> MYLSFYITDTKNKLIFQYLLGATAPSFKHLWTRVQSTCPQLLEDSSSDDYLDHSMVGRDLEVYKYFSVINKLNYWCLASTSKSKGPLDCFTFLETIDRILLEYFDKDKLSIKKIVNNYDRISLIFNCCVEAGEPNVSDMLYVNKIKEAVPERSDLSKFISSTAHNLQQAVQLPQQRQQQLQQNQISRGSNSLIENEEIVPWRTSRASKHENNELYVDLLETFHVVFEKKKSHLRLLTGSIHGIVDVRSYLNDNPLVAVKLNTMGNDIGIPSLHDCVEINDGVFSPSNITFIPPDGKFRLLEYSVDLSSQVKQSGVRMNSIGLMSLHFQNGLGKDS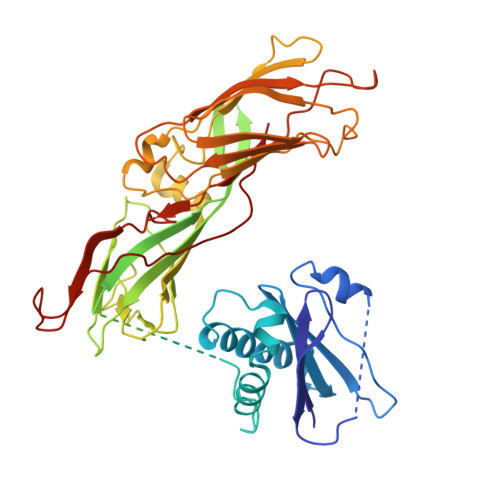DEFELSLNIENFKKVSQVDDLKIDLQFNVENADPNEIAYKIKILRNTHGRFENSIIMGQGQWIFDKSTATGTVPVLRGCIEYENTGPNFTKKVDLQTVSLEYSYIGQSASGIYVEAIDIVSGLTIGKNTKLYKGAKYKTQTGNFQVRL Aquaporins are water channels found in the cell membrane, where they allow the passage of water molecules in and out of the cells. In the kidney collecting duct, arginine vasopressin-dependent trafficking of aquaporin-2 (AQP2) fine-tunes reabsorption of water from pre-urine, allowing precise regulation of the final urine volume. Point mutations in the gene for AQP2 may disturb this process and lead to nephrogenic diabetes insipidus (NDI), whereby patients void large volumes of highly hypo-osmotic urine. Here we describe the structural and functional characterization of three AQP2 mutations associated with recessive NDI: T125M and T126M, situated close to a glycosylation site and A147T in the transmembrane region.

T125M and T126M are located in extracellular loop C, immediately downstream to an N-glycosylation site at Asn 123. In contrast to T125M, T126M can be glycosylated and is therefore able to enter the glycosylation-dependent quality control pathway. Specifically, a hydrophobic residue in position 3, as in the T126M mutant, correlated with increased glucosylation of glycopeptides. Hence, it seems plausible that T126M would be a better substrate for UGT than wild-type AQP2, despite being able to adopt the overall native fold. In contrast, T126M and A147T both showed significant amounts (30% and 50% respectively) of a population that most likely corresponds to the monomeric states, as well as the presence of higher oligomers and aggregates. Since the tetramers of both A147T and T126M were less stable than wild-type AQP2, this may play a role in the ER-retention of both these mutants. Overall, T126M gave crystals which diffracted to highest resolution, (~3–3.3 Å), followed by T125M (~3.7–4 Å). The T125M and T126M-structures are highly similar to wild-type AQP2, with root-mean-square deviations (RMSD) of 0.942 Å (929 Cα-atoms) for T125M and 0.322 (940 Cα-atoms) for T126M. Density for the methionine side chain could be observed in all monomers for T126M however this was not the case for T125M due to the lower resolution.

>[4x]GSELRSIAFSRAVFAEFLATLLFVFFGLGSALNWPQALPSVLQIAMAFGLGIGTLVQALGHISGAHINPAVTVACLVGCHVSVLRAAFYVAAQLLGAVAGAALLHEITPADIRGDLAVNALSNSTMAGQAVTVELFLTLQLVLCIFASTDERRGENPGTPALSIGFSVALGHLLGIHYTGCSMNPARSLAPAVVTGKFDDHWVFWIGPLVGAILGSLLYNYVLFPPAKSLSERLAVLKGLE8,8-diphenyl-2,3,4,8-tetrahydroimidazo[1,5-a]pyrimidin-6-amine 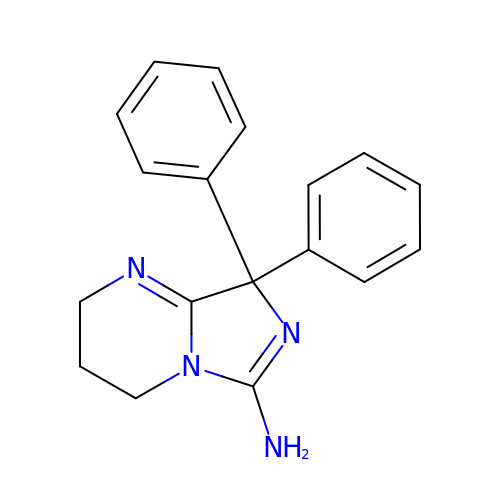| C18 H18 N4 | UFWSJOVQEPTPNE-UHFFFAOYSA-N(2Z,6E,10E)-2-fluoro-3,7,11,15-tetramethylhexadeca-2,6,10,14-tetraen-1-yl trihydrogen diphosphate | C20 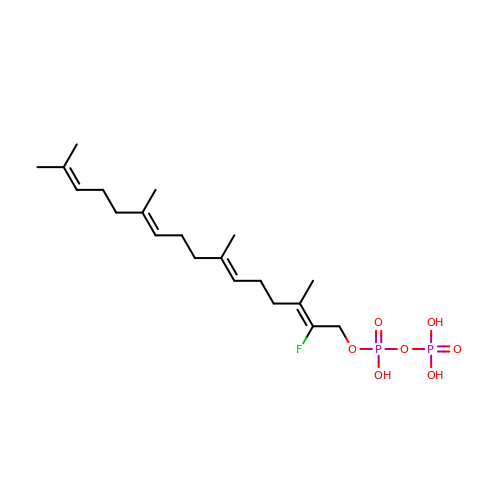H35 F O7 P2 | NZHGLLPGXYKTDW-HAQLZSGTSA-N>GPGSMIKIHTEKDFIKMRAAGKLAAETLDFITDHVKPNVTTNSLNDLCHNFITSHNAIPAPLNYKGFPKSICTSINHVVCHGIPNDKPLKNGDIVNIDVTVILDGWYGDTSRMYYVGDVAIKPKRLIQVTYDAMMKGIEVVRPGAKLGDIGYAIQSYAEKHNYSVVRDYTGHGIGRVFHDKPSILNYGRNGTGLTLKEGMFFTVEPMINAGNYDTILSKLDGWTVTTRDK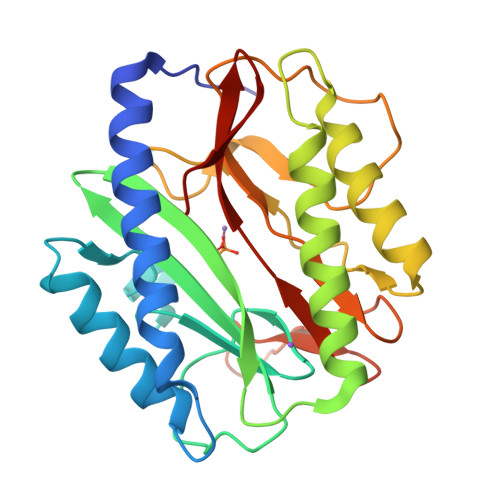SLSAQFEHTIGVTKDGFEIFTL[4x]> ASWSHPQFEKGASGAAESKPTPQSTFTGPIVVDPITRIEG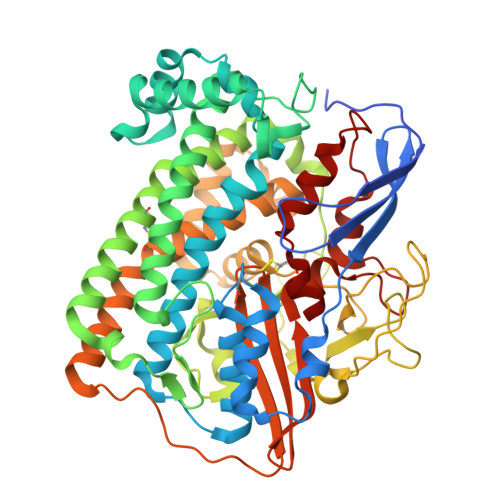HLRIMVEVENGKVKDAWSSSQLFRGLEIILKGRDPRDAQHFTQRACGVCTYVHALASSRCVDDAVKVSIPANARMMRNLVMASQYLHDHLVHFYHAHALDWVDVTAALKADPNKAAKLAASIAPARPGNSAKALKAVQDKLKAFVESGQLGIFTNAYFLGGHKAYYLPPEVDLIATAHYLEALHMQVKAASAMAILGGKNPHTQFTVVGGCSNYQGLTKDPLANYLALSKEVCQFVNECYIPDLLAVAGFYKDWGGIGGTSNYLAFGEFATDDSSPEKHLATSQFPSGVITGRDLGKVDNVDLGAIYEDVKYSWYAPGGDGKHPYDGVTDPKYTKLDDKDHYSWMKAPRYKGKAMEVGPLARTFIAYAKGQPDFKKVVDMVLGKLSVPATALHSTLGRTAARGIETAIVCANMEKWIKEMADSGAKDNTLCAKWEMPEESKGVGLADAPRGALSHWIRIKGKKIDNFQLVVPSTWNLGPRGAQGDKSPVEEALIGTPIADPKRPVEILRTVHAFDPCIACGVH>MTDTPFIRPDMKAFLEAIAAMAGPTLAEMTLEEARASYVALHGMADRPARELAVIRNLSCPGPAGDIPLRLYDARESREAGPVITFYHGGGFVIGDLDTHHNLCTEIAALMDLPVVAVDYRLAPEHPFPAAIEDCEAATRWVASSPSELGRTASGVIPIGDSAGGNATIVVSQLLGAKPADVPVVLQVPIFPLASDAVGSASLEAFAEGFVLTKASIEFFDTAYKADRADPRGFPILGDHTAAPPTIVATASLDPIRDSGRDYAKALVEAGRDVVYLE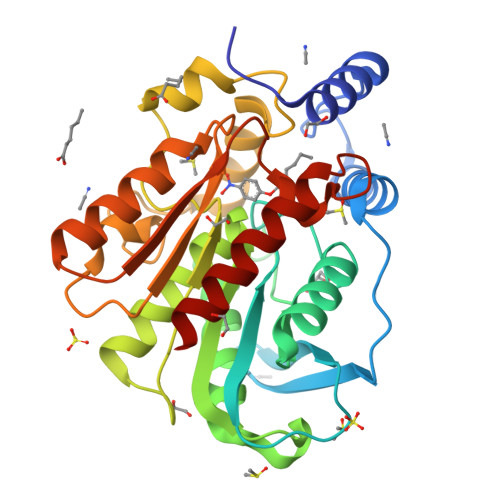MEGVTHSFTNIRAAVPSTQGDLERIIAAMKMMLGTA[4x]2,4-dibromo-6-{[(2-nitrobenzene-1-carbonyl)amino]methyl}phenyl 2-nitrobenzoate | C21 H13 Br2 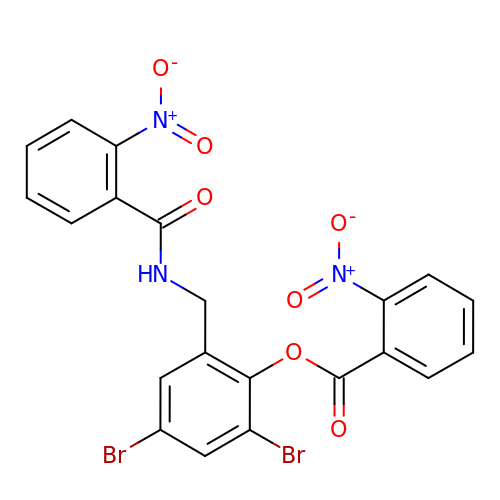N3 O7 | LZFWIBPLLYTTGG-UHFFFAOYSA-N The activity of β-ureidopropionase, which catalyses the last step in the degradation of uracil, thymine, and analogous antimetabolites, is cooperatively regulated by the substrate and product of the reaction. βUP in higher eukaryotes are nitrilase-like enzymes that use a tetrad of conserved active-site residues for catalysis of the CO–N bond cleavage. In human βUP (HsβUP), these catalytic residues correspond to C233, E119, K196, and E207. Substrate activation of human and rat enzymes is accompanied by a shift in their respective oligomer equilibria towards larger assemblies, which for HsβUP are primarily homooctamers.

For this purpose, we prepared grids for the C233S variant with 2 mM NCβA at pH 7.0, and for wild-type HsβUP without any ligands at pH 5.0. Only the latter sample resulted in micrographs that were of sufficient resolution and contained enzyme states larger than the dimer. Nevertheless, 3D classification showed that the sample was heterogeneous, consisting of tetramers, hexamers, and octamers. Map 1 has a resolution of ~3.0–3.5 Å for the two central HsβUP dimers, and >6 Å for the “outer” dimers, indicating that the latter region shows more variability. The structural model deposited in the PDB does in fact only consist of the two inner-most dimers, as the low resolution map obtained for the outer dimers prohibited a precise modelling of these parts. Out of the 384 amino acids comprising the HsβUP subunit, residues 3–300 and 307–368 are visible in the density map. In the cryo-EM structure reported here, the entrance loops as well as the N-terminal extension adopt conformations basically identical to those observed in the crystal structure of DmβUP. EL1 and EL2 are completely ordered, and EL3 partially. The lack of density for at least six residues at the very tip of this loop is indicative of their dynamic mobility. In the inner subunits involved in dimer–dimer interface formation, the last visible residue before the gap in density is H307, which was targeted in the here reported site-directed mutagenesis studies.

>MAGAEWKSLEECLEKHLPLPDLQEVKRVLYGKELRKLDLPREAFEAASREDFELQGYAFEAAEEQLRRPRIVHVGLVQNRIPLPANAPVAEQVSALHRRIKAIVEVAAMCGVNIICFQEAWTMPFAFCTREKLPWTEFAESAEDGPTTRFCQKLAKNHDMVVVSPILERDSEHGDVLWNTAVVISNSGAVLGKTRKNHIPRVGDFNESTYYMEGNLGHPVFQTQFGRIAVNICYGRHHPLNWLMYSINGAEIIFNPSATIGALSESLWPIEARNAAIANHCFTCAINRVGTEHFPNEFTSGDGKKAHQDFGYFYGSSYVAAPDSSRTPGLSRSRDGLLVAKLDLNLCQQVNDVWNFKMTGRYEMYARELAEAVKSNYSPTIVKE[4x]>[2x]MEYRLKAYYREGEKPSALRRAGKLPGLMYNRHLNRKVYVDLVEFDKVFRQASIHHVIVL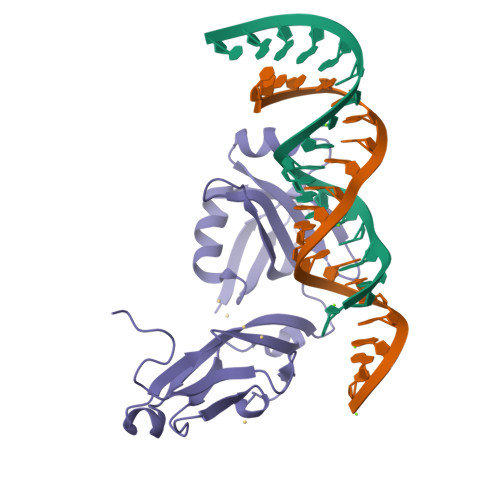ELPDGQSLPTLVRQVNLDKRRRRPEHVDFFVLSDEPVEMYVPLRFVGTPAGVRAGGVLQEIHRDILVKVSPRNIPEFIEVDVSGLEIGDSLHASDLKLPPGVELAVSPEETIAAVVPPEDVEKLAEEAAAEVAEPEVIKKGKEEEEE> ASKSKVDNQFYSVEVGDSTFTVLKRYQNLKPIGSGAQGIVCAAYDAVLDRNVAIKKLSRPFQNQTHAKRAYRELVLMKCVNHKNIISLLNVFTPQKTLEEFQDVYLVMELMDANLCQVIQMELDHERMSYLLYQMLCGIKHLHSAGIIHRDLKPSNIVVKSDCTLKILDFGLARTAGTSFMMTPYVVTRYYRAPEVILGMGYKENVDIWSVGCIMGEMVRHKILFPGRDYIDQWNKVIEQLGTPCPEFMKKLQPTVRNYVENRPKYAGLTFPKLFPDSLFPADSEHNKLKASQARDLLSKMLVIDPAK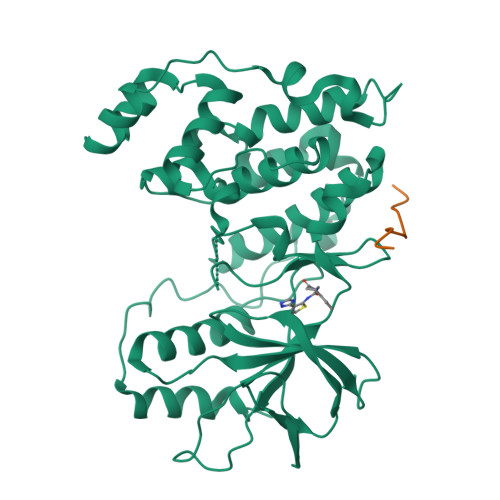RISVDDALQHPYINVWYDPAEVEAPPPQIYDKQLDEREHTIEEWKELIYKEVMNS;> RPKRPTTLNLF> MGHHHHHHSIETDRVSKEFIEFLKTFHKTGQEIYKQTKLFLEGMHYKRDLSIEEQSECAQDFYHNVAERMQTRGKVPPERVEKIMDQIEKYIMTRLYKYVFCPETTDDEKKDLAIQKRIRALRWVTPQMLCVPVNEDIPEVSDMVVKAITDIIEMDSKRVPRDKLACITKCSKHIFNAIKITKNEPASADDFLPTLIYIVLKGNPPRLQSNIQYITRFCNPSRLMTGEDGYYFTNLCCAVAFIEKLDAQSLNLSQEDFDRYMSGQTSPRKQMYKNLDLLSQLNERQERIMNEAKKLEKDLIDWTDGIARE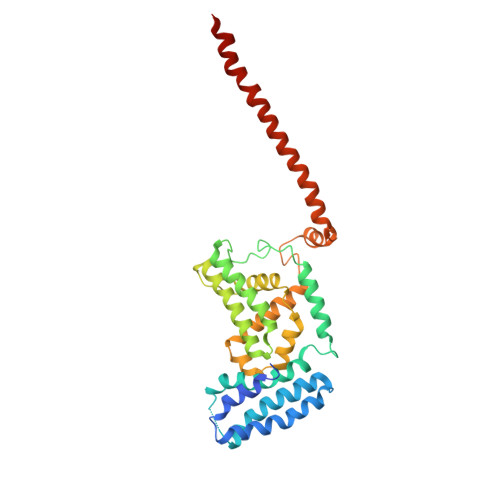VQDIVEK> GPHMPTEVILRGYRNAQHQYAAINHYEQIAGRICEDYPREPPVESRRYKSELRDPAFTHRRALTPEERAKVNRAMSGEHWVKVTFESAEAA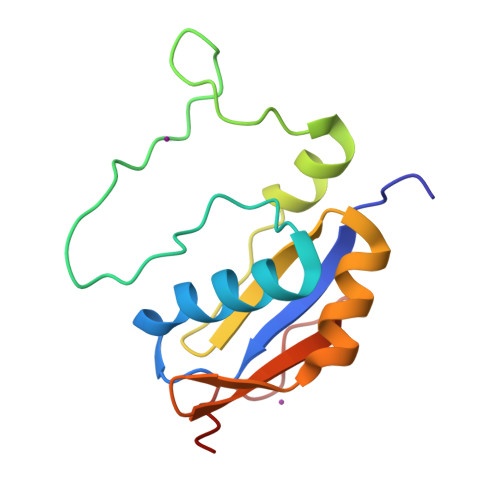DKAVYSSPQLIQGHLVYAEYYKGVPPAQDEAIPD2-{[2-(piperidin-1-yl)ethyl]amino}-3,5-dihydro-8H-imidazo[4,5-g]quinazolin-8-one 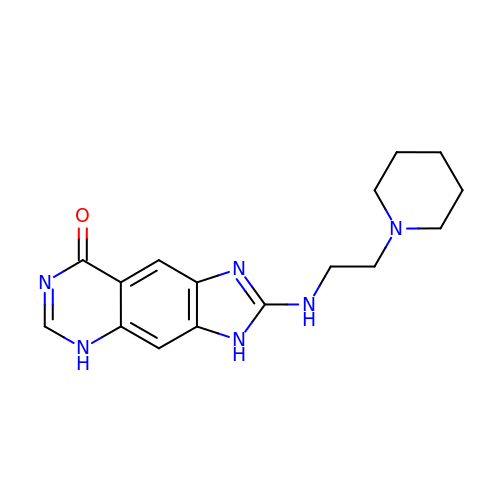| C16 H20 N6 O | NFLZHTAOFKJMSG-UHFFFAOYSA-N>[8x]MSLMKITSVDIIDVANDFASATSKWRPVVVKINTDEGISGFGEVGLAYGVGASAGIGMAKDLSAIIIGMDPMNNEAIWEKMLKKTFWGQGGGGIFSAAMSGIDIALWDIKGKAWGVPLYKMLGGKSREKIRTYASQLQFGWGDGSDKDMLTEPEQY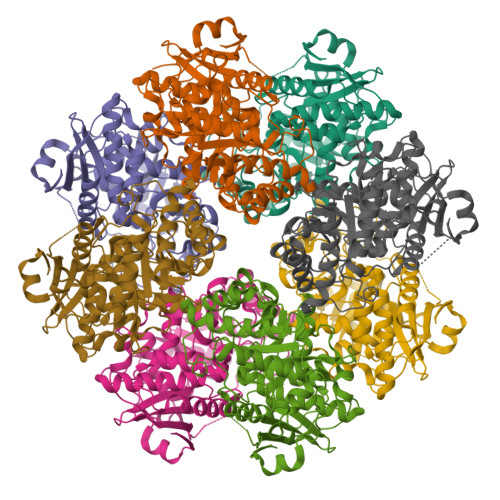AQAALTAVSEGYDAIKVDTVAMDRHGNWNQQNLNGPLTDKILRLGYDRMAAIRDAVGPDVDIIAEMHAFTDTTSAIQFGRMIEELGIFYYEEPVMPLNPAQMKQVADKVNIPLAAGERIYWRWGYRPFLENGSLSVIQPDICTCGGITEVKKICDMAHVYDKTVQIHVCGGPISTAVALHMETAIPNFVIHELHRYALLEPNTQTCKYNYLPKNGMYEVPELPGIGQELTEETMKKSPTITVKEGHHHHHH>[6x]MEEQIVPFYGKHQAGITTAHQTYVYFAALDVTAKEKSDIITLFRNWTSLTQMLTSGKKMSAEQRNQYLPPQDTGESADLSPSNLTVTFGFGPSFFEKDGKDRFGLKSKKPKHLAALPAMPNDNLDEKQGGGDICIQVCADDEQVAFHALRNLLNQAVGTCEVRFVNKGFLSGGKNGE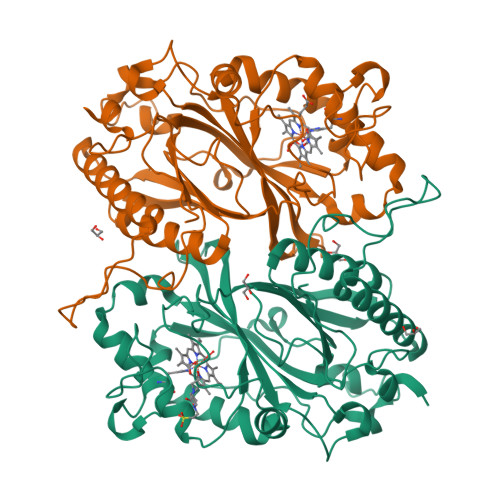TPRNLFGFKDGTGNQSTEDDSLMNSIVWVQSGEPDWMTGGTYMAFRKIKMFLEIWDRSSLKDQEDTFGRRKSSGAPFGQKKETDPVKLNQIPSNSHVSLAKSTGKQILRRAFSYTEGLDPKTGYMDAGLLFISFQKNPDNQFIPMLKALSAKDALNEYTQTIGSALYACPGGCKKGEYIAQRLLES> MADEIAKAQVARPGGDTIFGKIIRKEIPAKIIFEDDQCLAFHDISPQAPTHFLVIPKKHISQISAAEDADESLLGHLMIVGKKCAADLGLKKGYRMVVNEGSDGGQS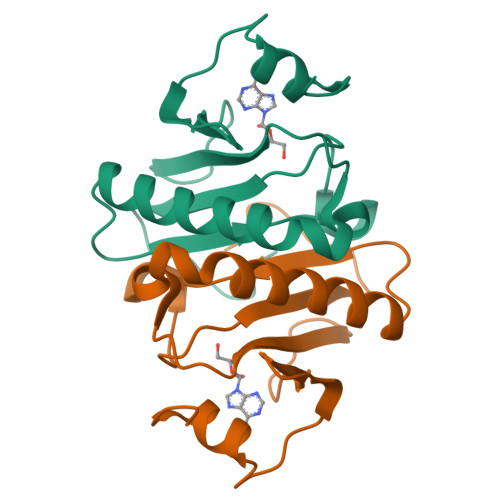VYHVHLHVLGGRQMNWPPG>[2x]GSHHHHHHGSAPMAEGGGQ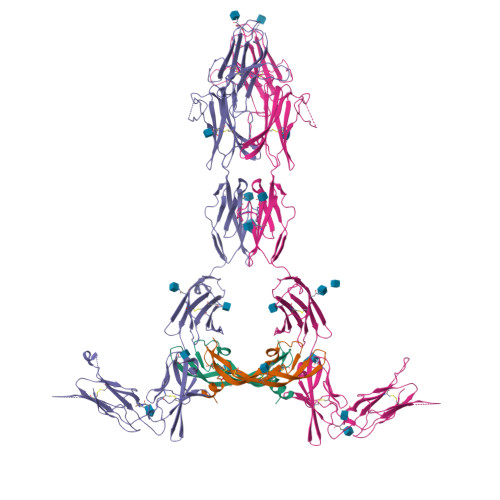NHHEVVKFMDVYQRSYCHPIETLVDIFQEYPDEIEYIFKPSCVPLMRCGGCCNDEGLECVPTEESNITMQIMRIKPHQGQHIGEMSFLQHNKCECRPKKDRARQENCDKPRR;>[2x]SKLKDPELSLKGTQHIMQAGQTLHLQCRGEAAHKWSLPEMVSKESERLSITKSACGRNGKQFCSTLTLNTAQANHTGFYSCKYLAVPTSKKKETESAIYIFISDTGRPFVEMYSEIPEIIHMTEGRELVIPCRVTSPNITVTLKKFPLDTLIPDGKRIIWDSRKGFIISNATYKEIGLLTCEATVNGHLYKTNYLTHRQTNTIIDVQISTPRPVKLLRGHTLVLNCTATTPLNTRVQMTWSYPDEKNKRASVRRRIDQSNSHANIFYSVLTIDKMQNKDKGLYTCRVRSGPSFKSVNTSVHIYDKAFITVKHRKQQVLETVAGKRSYRLSMKVKAFPSPEVVWLKDGLPATEKSARYLTRGYSLIIKDVTEEDAGNYTILLSIKQSNVFKNLTATLIVNVKPQIYEKAVSSFPDPALYPLGSRQILTCTAYGIPQPTIKWFWHPCNHNHSEARCDFCSNNEESFILDADSNMGNRIESITQRMAIIEGKNKMASTLVVADSRISGIYICIASNKVGTVGRNISFYITDVPNGFHVNLEKMPTEGEDLKLSCTVNKFLYRDVTWILLRTVNNRTMHYSISKQKMAITKEHSITLNLTIMNVSLQDSGTYACRARNVYTGEEILQKKEITIRDQEAIEGRHHHHHHHH> KRRWKKNFIAVSAANRFKKISSSGALENLYFQGEMVSPTKMIIASPAKETDTNLKHNNGIAASTTAAGHLNVFSNDNNCNNNNTTESFPKKRSLEALEAQQQQHLHEKKRARIERARSIEGAVQVSKGTGLKNVEPRVTPKELLEWQTNWKKIMKRDSRIYFDITDDVEMNTYNKSKMDKRRDLLKRGFLTLGAQITQFFDTTVTIVITRRSVENIYLLKDTDILSRAKKNYMKVWSYEKAARFLKNLDVDLDHL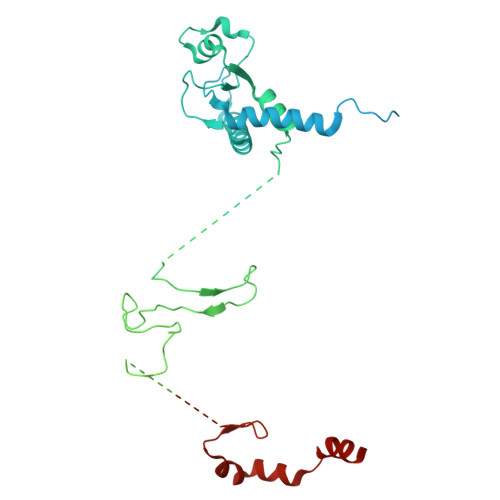SKTKSASLAAPTLSNLLHNEKLYGPTDRDPRTKRDDIHYFKYPHVYLYDLWQTWAPIITLEWKPQELTNLDELPYPILKIGSFGRCPFIGDRNYDESSYKRVVKRYSRDKANKKYALQLRALFQYHADTLLNTSSVNDQTKNLIFIPHTCNDSTKSFKKWMQEKAKNFEKTELKKTDDSAVQDVRNEHADQTDEKNSILLNETETKEPPLKEEKENKQSIAEESNKYPQRKELAATPKLNHPVLATFARQETEEVPDDLCTLKTKSRQAFEIKASGAHQSNDVATSFGNGLGPTRASVMSKNMKSLSRLMVDRKLGVKQTNGNNKNYTATIATTAETSKENRHRLDFNALKKDEAPSKETGKDSAVHLETNRKPQNFPKVATKSVSADSKVHNDIKITTTESPTASKKSTSTNVTLHFNAQTAQTAQPVKKETVKNSGYCENCRVKYESLEQHIVSEKHLSFAENDLNFEAIDSLIENLRFQI> 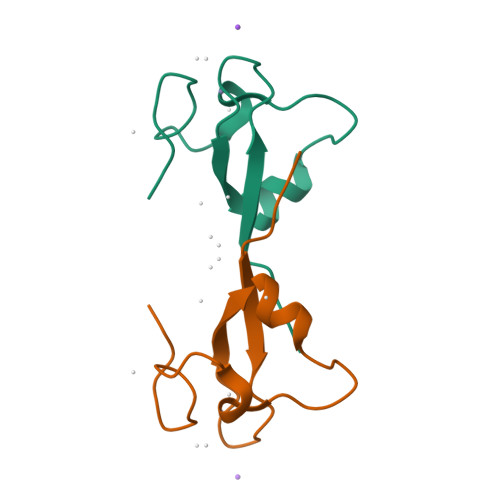GVENMYVNKVWVQCENENCLKWRLLSSEDSAKVDHDEPWYCFMNTDSRYNNCSISEEDD> GPHMSVEQTETAELPASDSINPGNLQLVSELKNPSGSCSVDVSAMFWERAGCKEPCIIT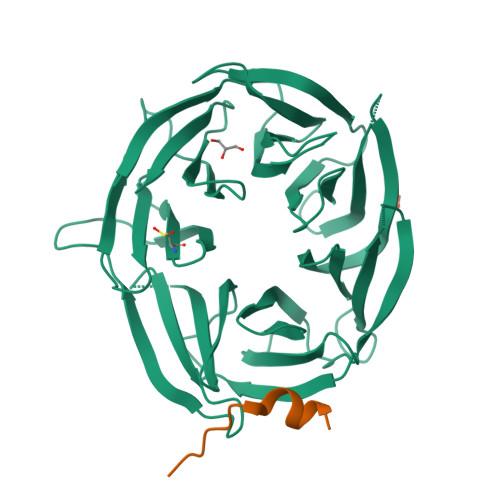ACEDVVSLWKALDAWQWEKLYTWHFAEVPVLQIVPVPDVYNLVCVALGNLEIREIRALFCSSDDESEKQVLLKSGNIKAVLGLTKRRLVSSSGTLSDQQVEVMTFAEDGGGKENQFLMPPEETILTFAEVQGMQEALLGTTIMNNIVIWNLKTGQLLKKMHIDDSYQASVCHKAYSEMGLLFIVLSHPCAKESESLRSPVFQLIVINPKTTLSVGVMLYCLPPGQAGRFLEGDVKDHCAAAILTSGTIAIWDLLLGQCTALLPPVSDQHWSFVKWSGTDSHLLAGQKDGNIFVYHYS;> KADLGPISLNWFEELSSEA> MGSSHHHHHHSSGGTENLYFQGHMILRPSMKLVKFRKGD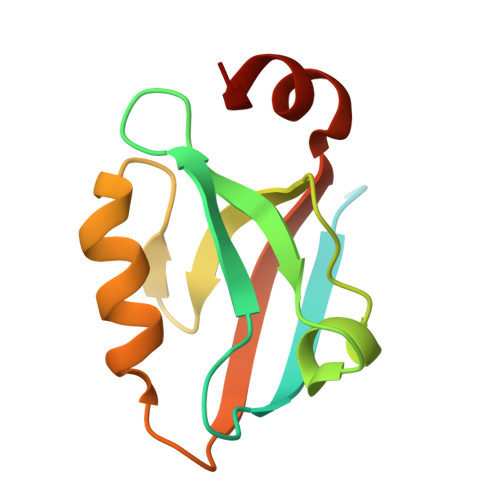SVGLRLAGGNDVGIFVAGVLEDSPAAKEGLEEGDQILRVNNVDFTNIIREEAVLFLLDLPKGEEVTILAQKKKDVYRRIVESDVG>[2x]GSHMSKAFDLVVIGAGSGGLEAGWNAATLYGKRVAVVDVQTSHGPPFYAALGGTCVNVGCVPKKLMVTGAQYMDHLRESAGFGWEFDGSSVKANWKKLIAAKNEAVLDINKSYEGMFNDTEGLDFFLGWGSLESKNVVVVRETADPKSAVKERLQADHILLATGSWPQMPAIPGIEHCISSNEAFYLPEPPRRVLTVGGGFISVEFAGI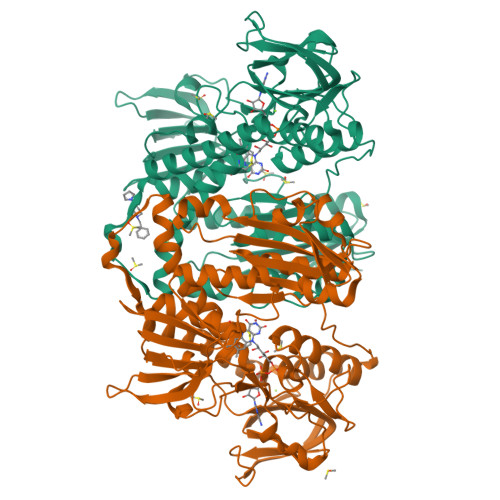FNAYKPPGGKVTLCYRNNLILRGFDETIREEVTKQLTANGIEIMTNENPAKVSLNTDGSKHVTFESGKTLDVDVVMMAIGRIPRTNDLQLGNVGVKLTPKGGVQVDEFSRTNVPNIYAIGDITDRLMLTPVAINEGAALVDTVFGNKPRKTDHTRVASAVFSIPPIGTCGLIEEVAAKEFEKVAVYMSSFTPLMHNISGSKYKKFVAKIVTNHSDGTVLGVHLLGDGAPEIIQAVGVCLRLNAKISDFYNTIGVHPTSAEELCSMRTPSYYYVKGEKMEKLPDSNL>[4x]GMNIEKTRFCINRKIAPGLSIEAFFRLVKRLEFNKVELRNDMPSGSVTDDLNYNQVRNLAEKYGLEIVTINAVYPFNQLTEEVVKKTEGLLRDAQGVGARALVLCPLNDGTIVPPEVTVEAI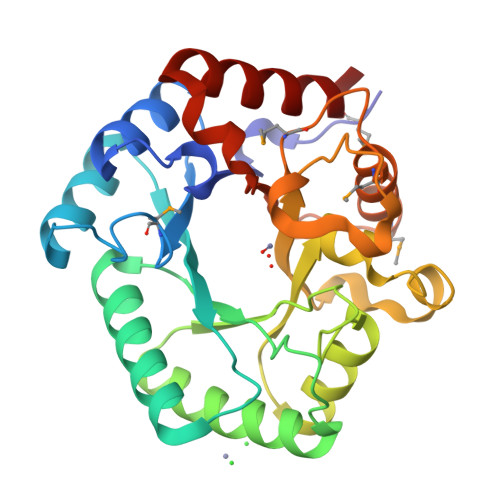KRLSDLFARYDIQGLVEPLGFRVSSLRSAVWAQQLIREAGSPFKVLLDTFHHHLYEEAEKEFASRIDISAIGLVHLSGVEDTRPTEALADEQRIMLSEKDVMQNYQQVQRLENMGYRGIYAFEPFSSQLASWSEAEIEEQINRSVSLLLQ> MVSTTQSRSLKAMGEEIWKNKTEKINTELFTLTYGSIVAQLCQDYERDFNKVNDHLYSMGYNIGCRLIEDFLARTALPRCENLVKTSEVLSKCAFK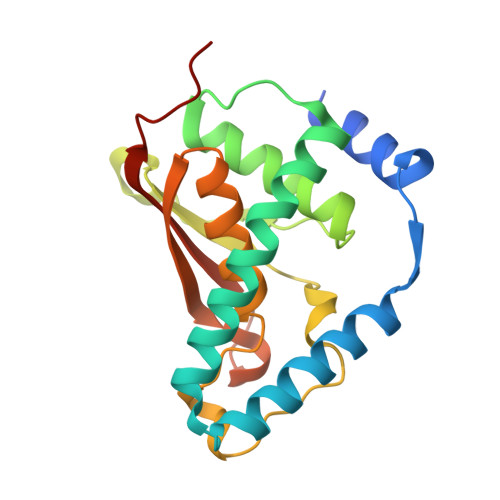IFLNITPNITNWSHNKDTFSLILDENPLADFVELPMDAMKSLWYSNILCGVLKGSLEMVQLDCDVWFVSDILRGDSQTEIKVKLNRILKDEIPIGED N-(tert-butoxycarbonyl)-L-phenylalanyl-N-{(1S)-1-[(R)-hydroxy(2-{[(2S)-2-methylbutyl]amino}-2-oxoethyl)phosphoryl]-3-methylbutyl}-3-(1H-imidazol-3-ium-4-yl)-L-alaninamide 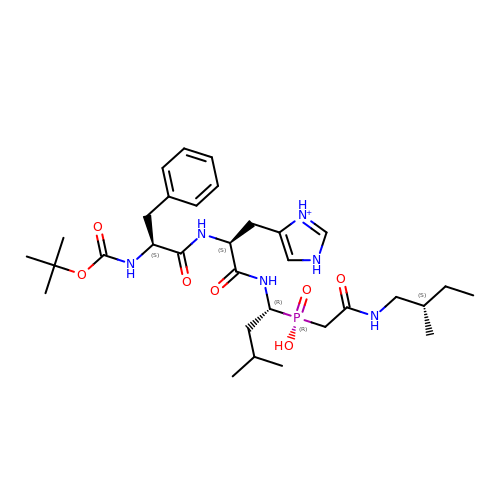| C32 H52 N6 O7 P | ZQDBBPUTYSTPQE-DYYCDWSUSA-O> MSALYFQNLPSRPANKENYTRLLLKHINPNNKYAINPSLPLPHNKLQISSQPLMLLDDQMGLLEVSISRSSKMTNQAFLTFVTQEEADRFLEKYTTTALKVQGRKVRMGKARTNSLLGLSIEMQKKKGNDETYNLDIKKVLKARKLKRKLRSDDICAKKFRLKRQIRRLKHKLRSRKVEEAEIDRIVKEFETRRLENMKSQQENLKQSQKPLKRAKVSNTMENPPNKVLLIQNLPSGTTEQLLSQILGNEALVEIRLVSVRNLAFVEYETVA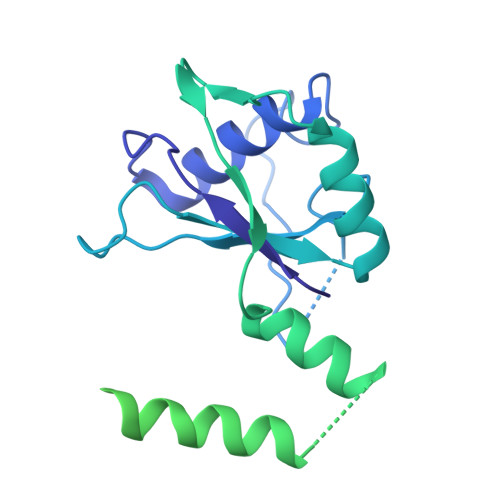DATKIKNQLGSTYKLQNNDVTIGFAKGRRIPGLINPWKRRWKKNFIAVSAANRFKKISSSGALDYDIPTTASENLYFQ> FHLTTRNGEPHMIVSRQEKGKSLLFKTEDGVNMCTLMAMDLGELCEDTLTYKCPLLRQNEPEDID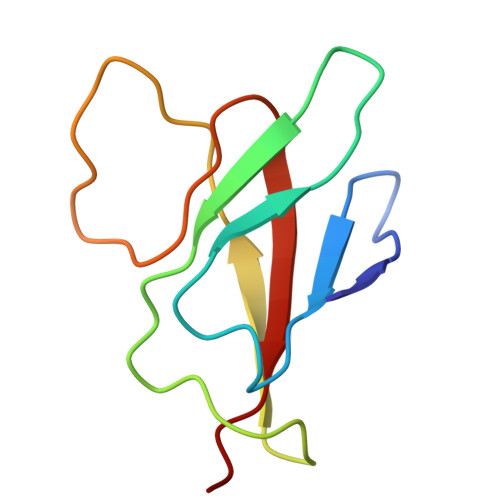CWCNSTSTWVTYGTCT> MKKQNDIPQPIRGDKGATVKIPRNIERDRQNPDMLVPPETDHGTVSNMKFSFSDTHNRLEKGGYAREVTVRELPISENLASVNMRLKPGAIRELHYHKEAEWAYMIYGSARVTIVDEKGRSFIDDVGEGDLWYFPSGLPHSIQALEEGAEFLLVFDDGSF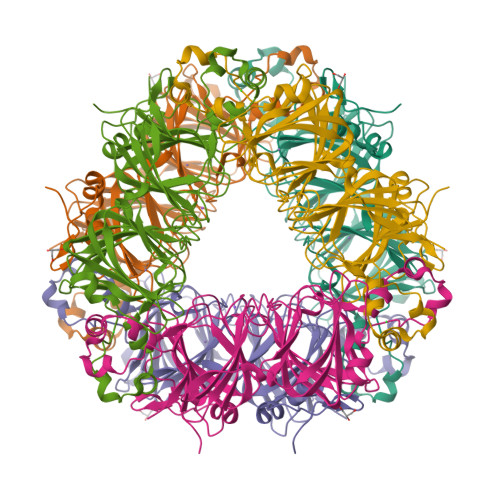SENSTFQLTDWLAHTPKEVIAANFGVTKEEISNLPGKEKYIFENQLPGSLKDDIVEGPNGEVPYPFTYRLLEQEPIESEGGKVYIADSTNFKVSKTIASALVTVEPGAMRELHWHPNTHEWQYYISGKARMTVFASDGHARTFNYQAGDVGYVPFAMGHYVENIGDEPLVFLEIFKDDHYADVSLNQWLAMLPETFVQAHLDLGKDFTDVLSKEKHPVVKKKCSK> VQRGYGNPIEASSYGLDLDCGAPGTPEAHVCFDPCQNYTLLDEPFRSTENSA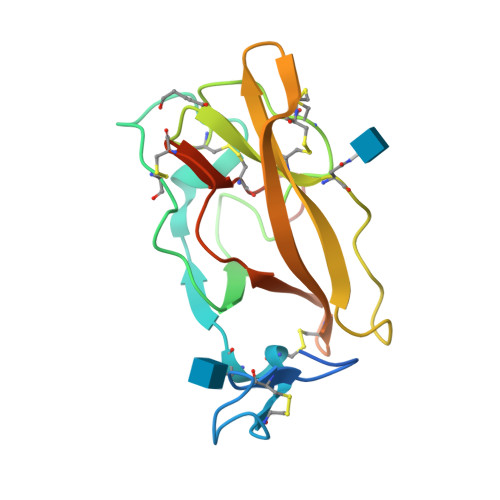GSQGCDKNMSGWYRFVGEGGVRMSETCVQVHRCQTDAPMWLNGTHPALGDGITNHTACAHWSGNCCFWKTEVLVKACPGGYHVYRLEGTPWCNLRYCTDPSHHHHHHHH>[4x]SNAMEGEHQYLNLVREILERGVKKDDRTGTGTLSIFGPQMRFSLRDDTIPVLTTKKIFWRGVVEELL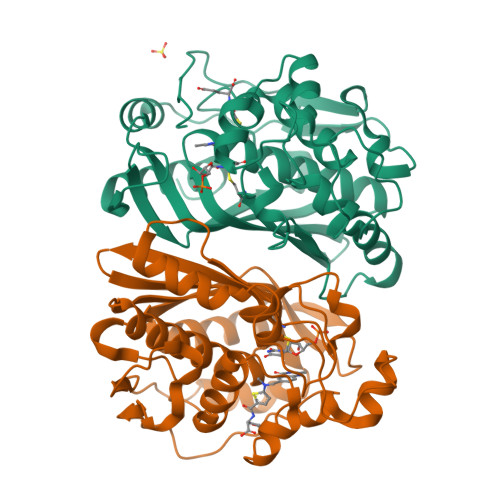WFIRGNTDAKELAKKKIHIWNANGSREFLDSRGLYDRAEGDLGPVYGFQWRHFGAEYDTCSSDYTGKGIDQLANILKTLRENPDDRRMIMTAWNPMDLHLMALPPCHMTAQFYVANGELSCQLYQRSGDVGLGVPFNIASYSLLTHLMASMVGLKPGEFILTLGDAHIYNTHIEVLKKQLCRVPRPFPKLRILMAPEKIEDFTIDMFYLEGYQPHSGNLQMKMAV PHYCOCYANOBILIN 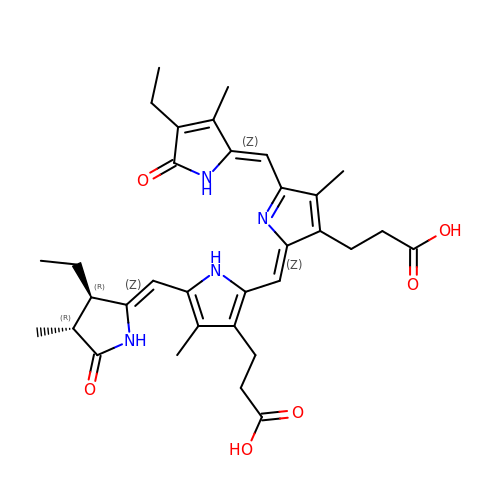| C33 H40 N4 O6 | VXTXPYZGDQPMHK-GMXXPEQVSA-N(3R,5R)-7-[3-(4-FLUOROPHENYL)-1-ISOPROPYL-8-OXO-7-PHENYL-1,4,5,6,7,8-HEXAHYDROPYRROLO[2,3-C]AZEPIN-2-YL]-3,5-DIHYDROXYHEPTANOIC 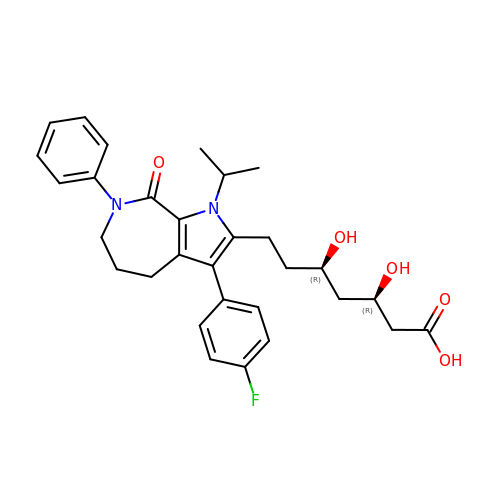ACID | C30 H35 F N2 O5 | OMBVEVHRIQULKW-DNQXCXABSA-N>[4x]KNRDMPLDSDVFRVPPGYNAPQQVHITQGDLVGRAMIISWVTMDEPGSSAVRYWSEKNGRKRIAKGKMSTYRFFNYSSGFIHHTTIRKLKYNTKYYYEVGLRNTTRRFSFITPPQTGLDVPYTFGLIGDL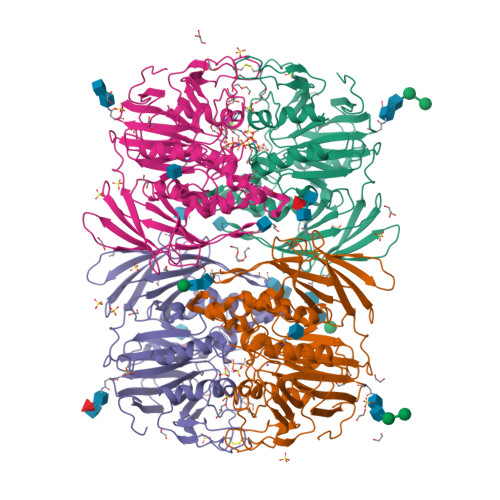GQSFDSNTTLSHYELSPKKGQTVLFVGDLSYADRYPNHDNVRWDTWGRFTERSVAYQPWIWTAGNHEIEFAPEINETEPFKPFSYRYHVPYEASQSTSPFWYSIKRASAHIIVLSSYSAYGRGTPQYTWLKKELRKVKRSETPWLIVLMHSPLYNSYNHHFMEGEAMRTKFEAWFVKYKVDVVFAGHVHAYERSERVSNIAYKITNGLCTPVKDQSAPVYITIGDAGNYGVIDSNMIQPQPEYSAFREASFGHGMFDIKNRTHAHFSWNRNQDGVAVEADSVWFFNRHWYPVDDST> IPIFLSVLQSIE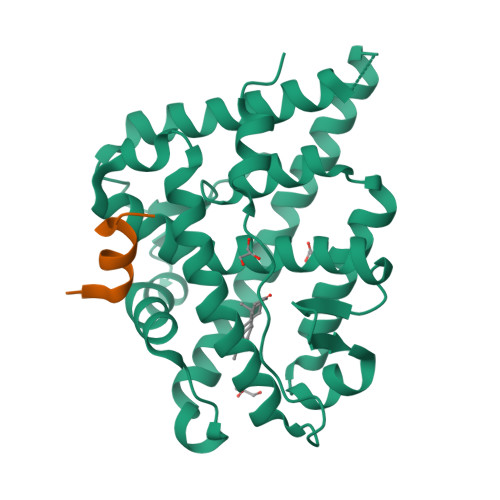PEVVYAGYDNTQPDTSASLLTSLNELGERQLVRVVKWAKALPGFRNLHVDDQMTLIQYSWMGVMVFAMGWRSYKNVNSRMLYFAPDLVFNEQRMQKSTMYNLCVRMRHLSQEFVWLQVTQEEFLCMKALLLFSIIPVEGLKNQKYFDELRMNYIKELDRVISFQGKNPTSSSQRFYQLTKLLDSLQDLVRKLHQFTFDTFVQSQSLSVEFPEMMSEIISAQVPKILAGMVKPLLFHKQ;> QALLRYLLDKDD>[2x]SGDMADAFGDELFSVFEGDSTTAAGTKKDKEKDKGKWKGPPGSADKAGKRFDGKLQSESTNNGKNKRDVDFEGTDEPIFGKKPRIEESITEDLSLADLMPRVKVQSVETVEGCTHEVALPAEEDYLPLKPRVGKAAKEYPFILDAFQREAIQCVDNNQSVLVSAHTSAGKTVCAEYAIALALREKQRVIFTS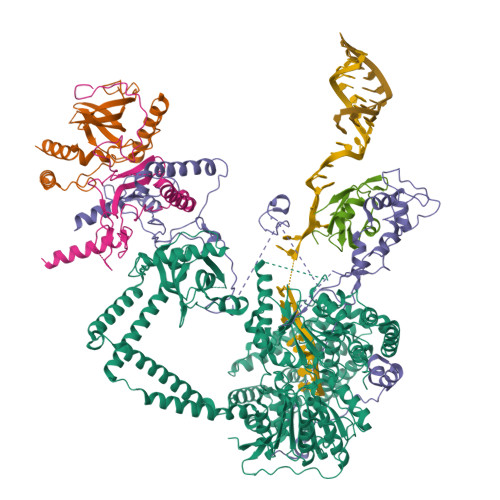PIKALSNQKYREMYEEFQDVGLMTGDVTINPTASCLVMTTEILRSMLYRGSEVMREVAWVIFDEIHYMRDSERGVVWEETIILLPDNVHYVFLSATIPNARQFAEWICHLHKQPCHVIYTDYRPTPLQHYIFPAGGDGLHLVVDENGDFREDNFNTAMQVLRDAGDLAKGDQKGRKGGTKGPSNVFKIVKMIMERNFQPVIIFSFSKKDCEAYALQMTKLDFNTDEEKKMVEEVFSNAIDCLSDEDKKLPQVEHVLPLLKRGIGIHHGGLLPILKETIEILFSEGLIKALFATETFAMGINMPARTVLFTNARKFDGKDFRWISSGEYIQMSGRAGRRGMDDRGIVILMVDEKMSPTIGKQLLKGSADPLNSAFHLTYNMVLNLLRVEEINPEYMLEKSFYQFQHYRAIPGVVEKVKNSEEQYNKIVIPNEESVVIYYKIRQQLAKLGKEIEEYIHKPKYCLPFLQPGRLVKVKNEGDDFGWGVVVNFSKKSNVKPNSGELDPLYVVEVLLRCSKESLKNSATEAAKPAKPDEKGEMQVVPVLVHLLSAISSVRLYIPKDLRPVDNRQSVLKSIQEVQKRFPDGIPLLDPIDDMGIQDQGLKKVIQKVEAFEHRMYSHPLHNDPNLETVYTLCEKKAQIAIDIKSAKRELKKARTVLQMDELKCRKRVLRRLGFATSSDVIEMKGRVACEISSADELLLTEMMFNGLFNDLSAEQATALLSCFVFQENSSEMPKLTEQLAGPLRQMQECAKRIAKVSAEAKLEIDEETYLSSFKPHLMDVVYTWATGATFAHICKMTDVFEGSIIRCMRRLEELLRQMCQAAKAIGNTELENKFAEGITKIKRDIVFAASLYL;>SGDMAAEVYFGDLELFEPFDHPEESIPKPVHTRFKDDDGDEEDENGVGDAELRERLRQCEETIEQLRAENQELKRKLNILTRPSGILVNDTKLDGPILQILFMNNAISKQYHQEIEEFVSNLVKRFEEQQKNDVEKTSFNLLPQPSSIVLEEDHKVEESCAIKNNKEAFSVVGSVLYFTNFCLDKLGQPLLNENPQLSEGWEIPKYHQVFSHIVSLEGQEIQVKAKRPKPHCFNCGSEEHQMKDCPMPRNAARISEKRKEYMDACGEANNQNFQQRYHAEEVEERFGRFKPGVISEELQDALGVTDKSLPPFIYRMRQLGYPPGWLKEAELENSGLALYDGKDGTDGETEVGEIQQNKSVTYDLSKLVNYPGFNISTPRGIPDEWRIFGSIPMQACQQKDVFANYLTSNFQAPGVKSGGAVDEDALTLEELEEQQRRIWAALEQAESVNSDSDVPVDTPLTGNSVASSPCPNELDLPVPEGKTSEKQTLDEPEVPEIFTKKSEAGHASSPDSEVTSLCQKEKAELAPVNTEGALLDNGSVVPNCDISNGGSQKLFPADTSPSTATKIHSPIPDMSKFATGITPFEFENMAESTGMYLRIRSLLKNSPRNQQKNKKASE[2x];> SGDEADRTLFVGNLETKVTEELLFELFHQAGPVIKVKIPKDKDGKPKQFAFVNFKHEVSVPYAMNLLNGIKLYGRPIKIQFRS>[6x]MRDMEFIEWYPRGYGVAFKVKRKILEEQSEYQKIEVYETEGFGKLLAIDGTVQLVTEGEKSYHEPLVHPAMLAHPNPRRVLIIGGGDGGAIREVLKHEEVEEVIMVEIDKKVIEISAKYIGIDG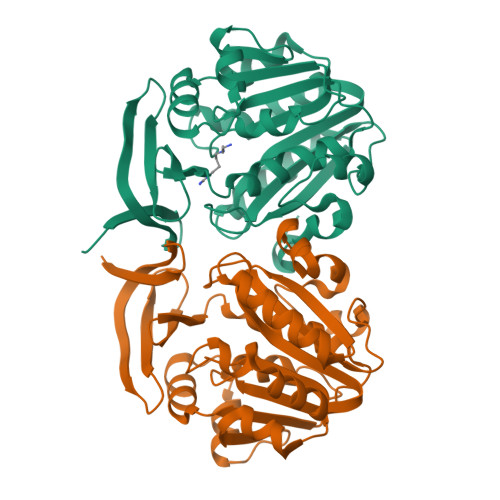GILEKMLSDKHEKGKLIIGDGVKFIEENSGFDVIIVDSTDPVGPAEMLFSEEFYKNAYRALNDPGIYVTQAGSVYLFTDEFLTAYRKMRKVFDKVYYYSFPVIGYASPWAFLVGVKGSIDFMKVDAEKGKKLGLEYYDPDKHETLFQMPRYIVQML(3R,4R)-3-[(1-carboxyethenyl)oxy]-4-hydroxycyclohexa-1,5-diene-1-carboxylic acid | C10 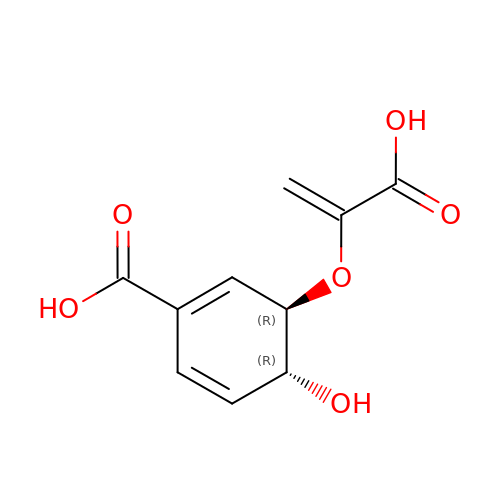H10 O6 | WTFXTQVDAKGDEY-HTQZYQBOSA-N>HHMEDKLIFAVDIIRHGDRTPIVALPTVNYQWQEGLGQLTAEGMQQEYKMGVAFRKKYIEESHLLPEHYEYGTIYVRSTDYARTLMSAQSLLMGLYPPGTGPTIPAGTSALPHAFQPIPVFSAPSKYDEVIIQQVDRKEREKLMEQYVFSTREWQQKNNELKDKYPLWSRLT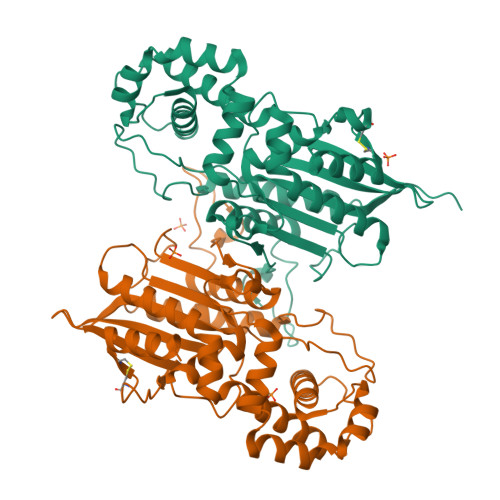GINIDNLGDLETVGHTLYIHQIHNAPMPEGLASNDIETIINSAEWAFMAQEKPQQIANVYSSKLMTNIADYLNSGSMKKSKLKYVLLSAHDTTIASVLSFLGAPLEKSPPYASNVNFSLYDNGANYYTVKITYNGNPVSIPACGGSVCELQQLINLVHDSKNS[4x]>GAMGMPSLKDEVSFENRVAETHKIRSKYPNRIPVVIERANRSNLPIIEKKKFLVPMNMLVGEFKFILHQHINQSAYGSNMKLFRERTIYLFVNNIVPKTGLLMQD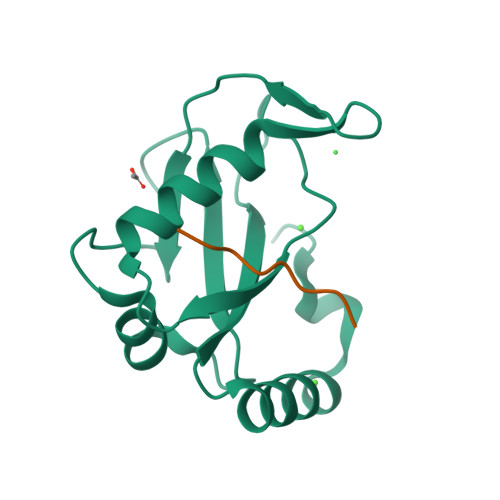LYEMYKDEDGYLYMEYSSESSLG[3x];>[3x]NDWLLPSY> EVTIEAVPPQVAEDNNVLLLVHNLPLALGAFAWYKGNTTAIDKEIARFVPNSNMNFTGQAYSGREIIYSNGSLLFQMITMKDMGVYTLD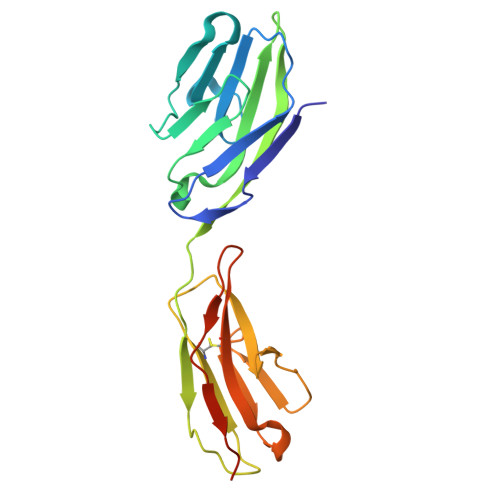MTDENYRRTQATVRFHVHQPVTQPFLQVTNTTVKELDSVTLTCLSNDIGANIQWLFNSQSLQLTERMTLSQNNSILRIDPIKREDAGEYQCEISNPVSVRRSNSIKLDIIFDPHHHHHH> MGIQGLAKLIADVAPSAIRENDIKSYFGRKVAIDASMSIYQFLIAVRQGGDVLQNEEGETTSHLMGMFYRTIRMMENGIKPVYVFDGKPPQLKSGELAKRSERRAEAEKQLQQAQAAGAEQEVEKFTKRLVKVTKQHNDECKHLLSLMGIPYLDAPSEAEASCAALVKAGKVYAAATEDMACLTFGSPVLMFHLTAS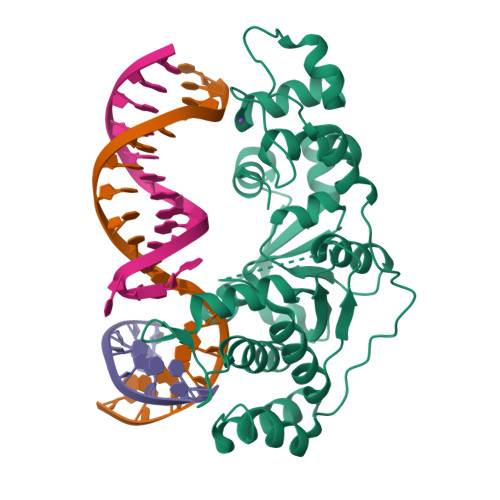EAKKLPIQEFHLSRILQELGLNQEQFVDLCILLGSDYCESIRGIGPKRAVDLIQKHKSIEEIVRRLDPNKYPVPENWLHKEAHQLFLEPEVLDPESVELKWSEPNEEELIKFMCGEKQFSEERIRSGVKRLSKSRQ5-methyl-1-(4-nitrophenyl)-2-oxo-2,5-dihydro-1H-pyrido[3,2-b]indole-3-carbonitrile | C19 H12 N4 O3 | 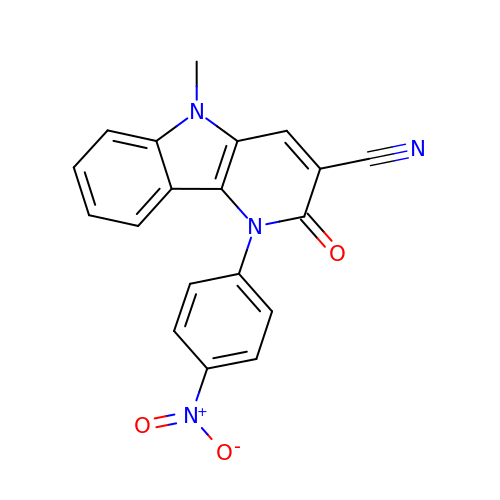TZEXGCXFOXXFKH-UHFFFAOYSA-N>GGEPAWDSPLRRVLAELNRIPSSRRRAARLFEWLIAPMPPDHFYRRLWEREAVLVRRQDHTYYQGLFSTADLDSMLRNEEVQFGQHLDAARYINGRRETLNPPGRALPAAAWSLYQAGCSLRLLCPQAFSTTVWQFLAVLQEQFGSMAGSNVYLTPPNSQGFAPHYDDIEAFVLQLEGRKLWRVYRPRVPTEELALTSSPNFSQDDLGEPVLQTVLEPGDLLYFPRGFIHQAECQDGVHSLHLTLSTYQRNTWGDFLEAILPLAVQAAMEENVEFRRGLPRDFMDYMGAQHSDSKDPRRTAFMEKVRVLVARLGHFAPVDAVADQRAKDFIHDSLPPVLTDRER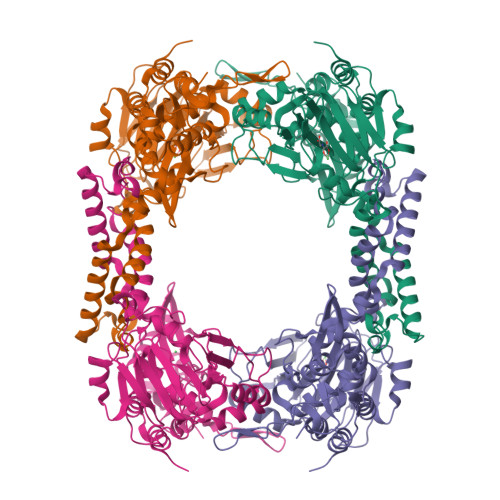ALSVYGLPIRWEAGEPVNVGAQLTTETEVHMLQDGIARLVGEGGHLFLYYTVENSRVYHLEEPKCLEIYPQQADAMELLLGSYPEFVRVGDLPCDSVEDQLSLATTLYDKGLLLTKMPLALN[4x]> GSHMASPNGQTKPLPALKLALEYIVPCMNKHGICVVDDFLGKETGQQIGDEVRALHDTGKFTDGQLVSQKSDSSKDIRGDKITWIEGKEPGCETIGLLMSSMDDLIRHCNGKLGSYKINGRTKAMVACYPGNGTGYVRHVDNPNGDGRCVTCIYYLNKDWDAKVSGGILRIFPEGKAQFADIEPKFDRLLFFWSDRRNPHEVQPAYATRYAITVWYFDADERARAKVKYLTGE;> XYVWLTDTWVLSRT;> DLDLEMLAPYIPMDDDFQL

The degradation of HIFα subunits is promoted by post-translational hydroxylation of prolyl-residues located in its N/C-terminal oxygen dependent degradation domains (NODD and CODD). These dioxygen-sensitive reactions are catalysed by 2-oxoglutarate (2OG) and Fe(II) dependent prolyl hydroxylases (PHD 1–3 in humans). The human PHDs catalyse hydroxylation of prolyl-residues within the N/C terminal ODDs of HIF-1/2/3α and are negative regulators of the transcriptionally regulated hypoxic response.

Following screening for cyclic peptides (CPs) binding to PHD2 via a modified mRNA display methodology, we identified a 14-mer cyclic peptide thioether (3C) that promotes crystallization of the catalytic domain of PHD2, whilst still enabling a catalytically productive substrate binding mode. Pleasingly, we also discovered that 3C enables rapid crystallization of cPHD2 in the presence of 2OG (or NOG) and the substrate, HIF-1α CODD (aa 556–574), in the P21212 form. Although binding of 3C induces structural changes in cPHD2 C-terminal residues (400–404) that form part of the C-terminal helix (α4), 3C binding allows protein–protein interactions between the cPHD2 C-terminus and the HIF-α substrate, consistent with the catalytic activity observed in the presence of 3C. Binding of 3C at the interface of two symmetry related PHD2 monomers likely promotes contacts productive for crystallization in part via projecting part of the C-terminal helix α4 (aa 400–404) away from the active site, in a manner that maintains interactions with substrates that are required for catalysis.> AMAAAPDFSSALSLRSSTATSQQNSLSTNIFASGDVSPQTPTPPQADEKTEDCLAIINKLRSENLKDLLGTLAKAEDTEVTESLKAIKIEEPASPTAPKIAVTLAGSNVDTCESGEGANAKKYPGLVIPFPHDTEFNCNALIQATYTAGLDHLKQSNFEPSTGTYDVENAPFNNVNASNVAFLLSEKSKKVSCAATKDCKAGHDVLFCYFIDPLRKEDKPFTAELYNALWGLEALEHHHHHH

Eimeria tenella causes caecal coccidiosis in chickens and has a SAG family with over 80 members making up 1% of the proteome. In addition, a further 20 regions of the E. tenella genome were identified as encoding sag pseudogenes. These EtSAGs comprise a cysteine-rich ectodomain of ~300 residues, including an N-terminal signal sequence and a site at the C-terminus for a glycosylphosphatidylinositol (GPI) anchor for membrane attachment. We have solved the structure of a representative E. tenella SAG, EtSAG19, revealing that, despite a low level of sequence similarity, the entire Eimeria SAG family is unified by its three-layer αβα fold which is related to that of the CAP superfamily. While it has been established that SAGs are expressed on the surface of Eimeria parasites, it is currently unknown whether these proteins are involved in aspects of cell adhesion, invasion or in some other process.

The structure of E. tenella SAG19 was solved by sulphur-SAD to 1.32 Å to reveal that the protein adopts an αβα sandwich fold, and providing an experimental three-dimensional model for the protein. EtSAG19 comprises a four-stranded, anti-parallel, β-sheet surrounded by six α-helices with an additional 310 helix and 12 loops, 10 of which connect regions of regular secondary structure together with two additional loops to the N- and C-terminus. The loop regions in EtSAG19 are extensive and account for ~50% of the entire structure with some of the loops being large with, for example, 20 residues in the loop between helix III and strand B (L5). As predicted, given its cysteine content, EtSAG19 contains three disulphide bonds, SS1 (connecting C67 and C152), SS2 (connecting C126 and C213) and SS3 (connecting C207 and C222). The structure also contains three cis peptides, two of which involve proline (E105-P106 in loop L4 that links helix II to helix III and, A184-P185 in loop L7 leading to the 310 helix, helix V’). The third cis peptide is more unusual in that it is a rare non-proline cis peptide between I225 and D226 in loop L11 linking strand D to helix VI, forming a tight turn in the structure. Analysis of the structure showed that these conserved residues are located within the buried core of the protein, and broadly lie in three clusters, one (cluster 1) on one face of the central β-sheet with the remaining two clusters (clusters 2 and 3) found on the opposite face. Analysis of the structure shows that these sidechains participate in an intricate network of hydrogen bonds that help to pin the extended loop L3 found between αI and αII to αI and the C-terminus of αV. Therefore, the conservation of N72 and the buried arginine, R75, are particularly important in preserving the overall 3D structure of the protein, and, in our view, act as a fingerprint for the fold.> MPQIFSRKTNRLPALSLAGSVFGGVLAVFLVWYYFSPEFYEVGYAPPYSHRIHVGKLGLDCRYCHNWVEVSDKANIPPTQTCINCHSQILTDSPRLQAVRDSWATDRSIEWVKVHHLPDYAHFSHASHVNNGVGCETCHGRIDQMDVVRLVEPLSMGWCLECHRQPELYLRPQSEITTMGYQPPADYIERNLERIRKEGIRPPTNCSACHY;> MIELPVVNPDGAETPGSGKRLWRSTADLRRDPEWVKLAHDEFMPGVAEPPSGTSRRQFLQIMGASMALAGLTACRRPVEKILPYVRQPEEIIPGIPLYYATAMPFRGSVRPLLVESHEGRPTKIEGNPDHPLSRGATGVFEQASLLNLYDPDRSQQVLRKGEPASWGDFVQFARSLAAEAGTKRLAVLCEPSSSPTLAALRRELERRYAQVRWVTYRPEGDDHEALGLQQAFGRPVRARYRFSEARVIVSLDADFLGPTDRNFVENTREFAASRRMERPEDEISRLYVIESTYTVTGGMADHRLRLRAGDIPAFAAALAAELGVGELREAGARFAGHPYVVEIARDLRAAGARGVVLAGETQPPAVHALCAVINDLLGSLGRTVILHALDEPATAQHAALAELVQAMQAGAVDALLLLNVNPVYDAPAALGFAEALAQVPEVIHLGLHVDETARRSTWHLPSTHYLEAWGDGRAYDGTLSVIQPLIAPLYEAAHSPLEVLALLATGEEQSAYDLVRNTWRRLLAGRGAFEQAWQRVLHDGFLPDSGYPTVSLRPNRQALADWPQAAE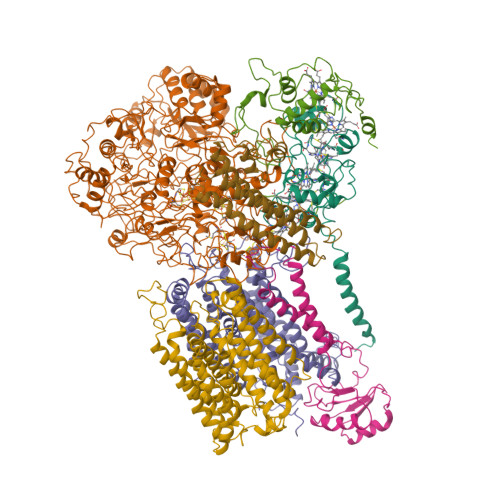GGLEVVFRLDPTVLDGSFANNAWAQELPDPITKIVWDNVAILSPKTAAALGVKAEYHKGVYIADVIELSLDGRAVELPVWVLPGHPDDSITVYLGYGREITSTRPERKTPFFDLDDYTDIYGHGAIATGVGVNVAPLRRPDNTWVAYGAQVRKTGRTYKIVTTQDHGSMVGRPLVRLATVEEFRKNPDFAKEAEPPLEGLEPWDQYPTLWEENHPSKQPAFQDSDYYRNQWAMVIDLNACTGCNACIVACDSENNIPMVGKNEVGRGREMHWLRIDRYFVSDEAHADDPQIVVQPVPCMHCENAPCESVCPVAATVHSPDGLNEMVYNRCIGTRYCSNNCPYKVRRFNWFNWVKTLPIQVQMAQNPDVTVRFRGVMEKCTYCVQRIREAQRQANIEKRPLRDGEVKTACQQACPAEAITFGDLNDPNNAVVKQRQNARRYEMLAALNVKPRTSYLARITNPNPRLLEQEPVA;> MAHATKDLSALARTDEEVLVQGGLTFHDITELVAQHTEKKTPKAWWAAFSVAFLGMLTLVAMLAYQVWNGVGVWGNNIPVGWGWPIVNFVFWVGIGHAGTLISAILFLFRQRWRTSINRAAEAMTIFAVICALIFPTFHVGRVWAIYWTLPIPNQMEMWPQFKSPLLWDVFAVSSYFIVSLVFWYVGLIPDLATLRDRAALMGRRLRAKILGFFALGWCGANRHWRNYEKVYMLLAGLATPLVLSVHSVVSFDFAVSIIPGWHTTIFPPYFVAGAIFSGFAMVVTLMVIARKAYGLENVITIDHLEKMNIIMLVTGTMVGFAYITEFFIAWYSGVPYEQYAFINRATGPYAWAYWTMMSCNLIFPQFFWIKKLRRNIPFMFIASIVVNIGMWFERFVITITSLHRDYLPSSWDYFVPTWVDVLTLIGSFGLFFTLFLLFLRFVPMVAIAEVKGVLPEADPHFYETHGDGHSRPAEVQVNRGRSS;> MLKELLRSLKASMGIYEARDGSIYGLLAEFSDPAALLHAARQVRKAGYRHFDAHSPFPIHGMDEAMGLGNSKVAFITFFTGTIAGFALAWWMQWWMGAVDYPLNISGKPFFALPPSVPIIFELTILFSALAGVATMLALNGLPRPYNPLFYSKNFMRVTDDGFFLFVAASDPKFDPTATRQLLEQLGGYNIEVIEDRGEEDVTPATAPAAEAAVTTS;> MQNITAMPRTIWTGLLLGLLLAGCRGMISSKPPVHPNLNMDFQEKFEAQELNPFFADRRAMRPPVPGTVPRGLLKEDTPFYFGKTADGAYVERIPVAVTPELVARGRERYNIYCAVCHGQAGDGQGIIMRGNYGYTPAPSFHDDRLRNVEDGYIFDVISHGVRNMPAYGHQIPVADRWAIVAYVRALQRSQHATAADVPEEVRARLQGE;> MAEVKANGFPGWLLDPLRPTREKAEPRYRLPEDVRIWAVPLAIGVGLLIVSLVGWAIDARQFYFSYLVGWTFCLTLALGSLFFVMIQHLTRAQWVVAVRRLPEALVWTFPVLIVLFIPILFGLHDLYHWTHHELYDPSSPEYDPILAGKHAYLNVPFFLVRIAFYFFIWTLLAYKLYTLSVRQDVDPDPSIPAQQRKVSAWGMPLYGVTVAFASYDFLMSLDPHWYSTIFGVYFFAGSFFVALGFITTCYAILVRRGTLQGIVRAPHFQDLGKLMFGFTAFWAYIAFSQYMLIWYGNLPEETLWYRHRLEHGWEVLSQVLIWGHFVLPFLILLPWAAKRTPVLVGTMGIWFAIIHWIDLFWVAMPVLHTEHMTFHWLDVTCWLGLFGVVVGLFFYRISRHSLVPQNDPYLARSLALH;> MKRYPGLIGLLVVLVSVAGCRFYGYPGGVALTLAQIEAASEQVAQDLEQALAELEALRLLARRDETLAPYVAQYEAILEAHQQAVLEFEHWKEQVAAHPGDYRRANRTLGAITARHEALLQQYADVAWAVAQHVNPALLARAYTSSGPRFFFYVVPPQYARQVNEQAVPPLQVVRYLAAQLS3-(1H-indol-3-yl)-N-{[(2R,3R,4R,5R,6S)-3,4,5-trihydroxy-6-methylpiperidin-2-yl]methyl}propanamide | C18 H25 N3 O4 | 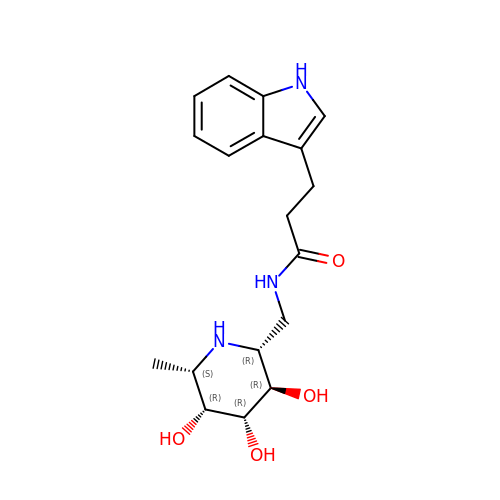QUTVJEWHGONWDR-YCIWZXPNSA-N> ATLDSWLSNEATVARTAILNNIGADGAWVSGADSGIVVASPSTDNPDYFYTWTRDSGLVIKTLVDLFRNGDTDLLSTIEHYISSQAIIQGVSNPSGDLSSGGLGEPKFNVDETAYTGSWGRPQRDGPALRATAMIGFGQWLLDNGYTSAATEIVWPLVRNDLSYVAQYWNQTGYDLWEEVNGSSFFTIAVQHRALVEGSAFATAVGSSCSWCDSQAPQILCYLQSFWTGSYILANFDSSRSGKDTNTLLGSIHTFDPEAGCDDSTFQPCSPRALANHKEVVDSFRSIYTLNDGLSDSEAVAVGRYPEDSYYNGNPWFLCTLAAAEQLYDALYQWDKQGSLE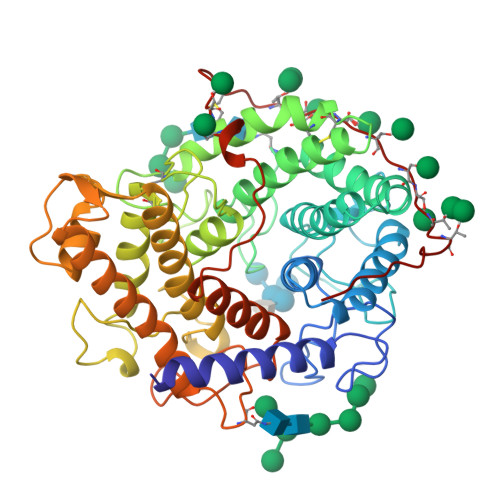ITDVSLDFFKALYSGAATGTYSSSSSTYSSIVSAVKTFADGFVSIVETHAASNGSLSEQFDKSDGDELSARDLTWSYAALLTANNRRNSVVPPSWGETSASSVPGTCAATSASGTYSSVTVTSWPSIVATG1-CHLORO-2,2,2-TRIFLUOROETHYL DIFLUOROMETHYL ETHER | C3 H2 Cl F5 O | 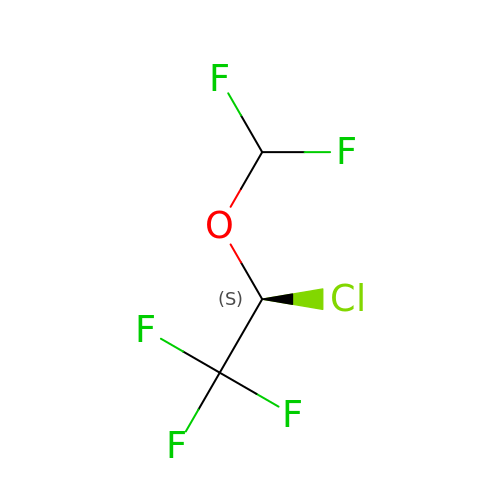PIWKPBJCKXDKJR-PVQJCKRUSA-N>HHHHHHHHHHSSGHIEGRHMKPSFSPRNYKALSEVQGWKQRMAAKELARQNMDLGFKLLKKLAFYNPGRNIFLSPLSISTAFSMLCLGAQDSTLDEIKQGFNFRKMPEKDLHEGFHYIIHELTQKTQDLKLSIGNTLFIDQRLQPQRKFLEDAKNFYSAETILTNFQNLEMAQKQINDFISQKTHGKINNLIENIDPGTVMLLANYIFFRARWKHEFDPNVTKEEDFFLEKNSSVKVPMMFRSGIYQVGYDDKLSCTI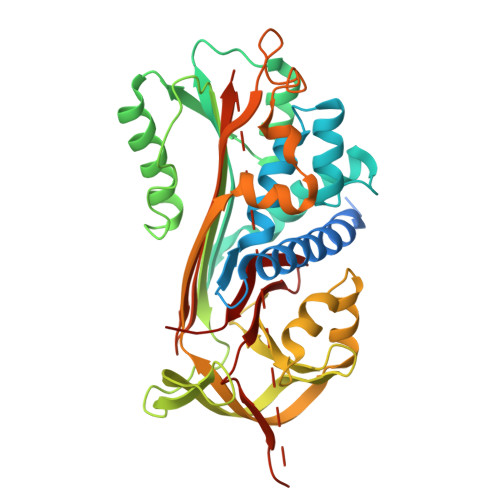LEIPYQKNITAIFILPDEGKLKHLEKGLQVDTFSRWKTLLSRRVVDVSVPRLHMTGTFDLKKTLSYIGVSKIFEEHGDLTKIAPHRSLKVGEAVHKAELKMDERGTEGAAGTGAQTLPMETPLVVKIDKPYLLLIYSEKIPSVLFLGKIVNPIGK[2x]> THVDLGLASANVDFAFSLYKQLVLKAPDKNVIFSPLSISTALAFLSLGAHNTTLTEILKGLKFNLTETSEAEIHQSFQHLLRTLNQSSDELQLSMGNAMFVKEQLSLLDR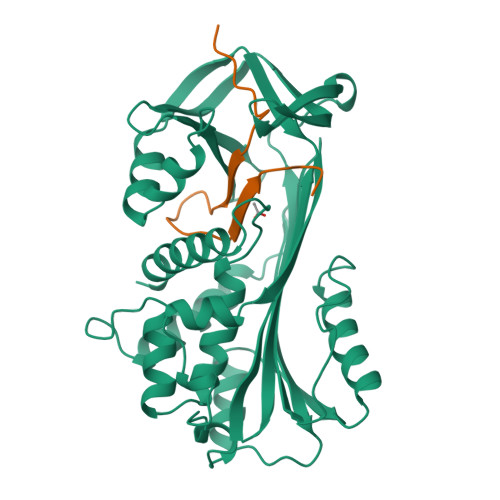FTEDAKRLYGSEAFATDFQDSAAAKKLINDYVKNGTRGKITDLIKDLDSQTMMVLVNYIFFKAKWEMPFDPQDTHQSRFYLSKKKWVMVPMMSLHHLTIPYFRDEELSCTVVELKYTGNASALFILPDQDKMEEVEAMLLPETLKRWRDSLEFREIGELYLPKFSISRDYNLNDILLQLGIEEAFTSKADLSGITGARNLAVSQVVHKAVLDVFEEGTEASRATAVKITLL;> VETGTIVRFNRPFLMIIVPTDTQNIFFMSKVTNPKQA> MTSKETFTHYQPQGNSDPA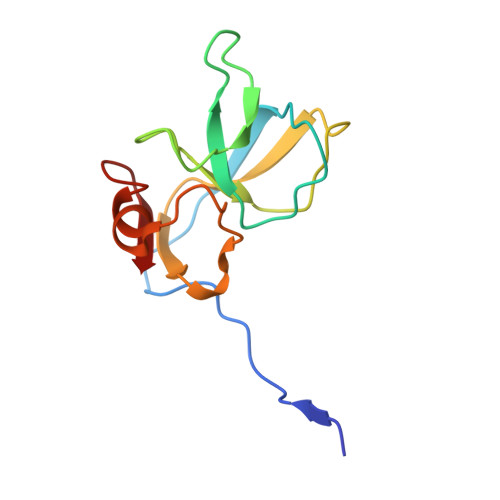HTATAPGGLSAKAPAMTPLMLDTSSRKLVAWDGTTDGAAVGILAVAADQTSTTLTFYKSGTFRYEDVLWPEAASDETKKRTAFAGTAISIV4-[3-CHLORO-4-({[(2,4-DICHLOROBENZOYL)AMINO]CARBONYL}AMINO)PHENOXY]BUTANOIC ACID | C18 H15 Cl3 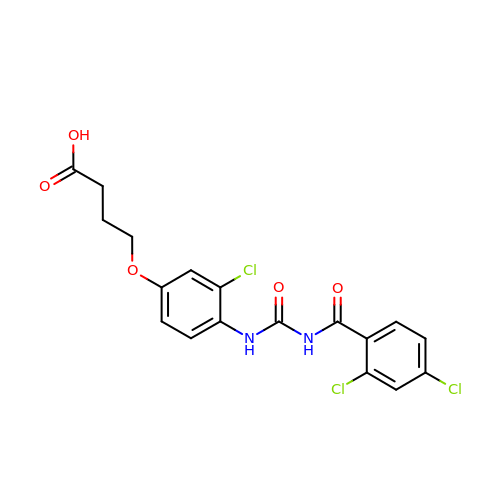N2 O5 | FYQVFMLCZJZZEM-UHFFFAOYSA-N>[4x]ADKELKFLVVDKFSTMRRIVRNLLKELGFNNVEEAEDGVDALNKLQAGGYGFVISDWNMPNMDGLELLKTIRADGAMSALPVLMVTA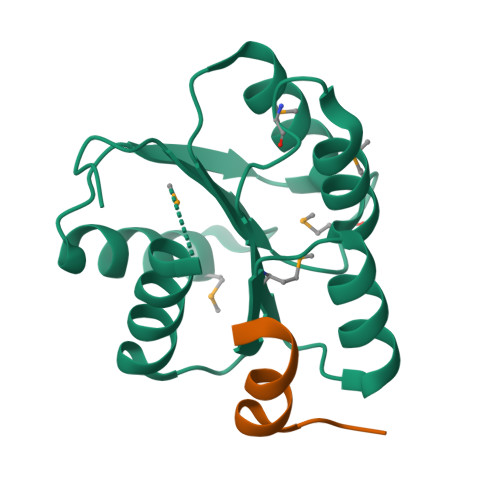EAKKENIIAAAQAGASGWVVKPFTAATLEEKLNKIFEKLGM;>MGDSILSQAEIDALLN[2x]> GSARNHTEDNSTEYYDYEEARCACPARHLNNTNGTVLKLLGCHYFCNGTLCTAPDGYPCYNLTAQQVRTLTTYPNTSCAVGVCMKGTCVKNGTMEQCFKTP;> ARGTNVGRECCLEYFKGAIP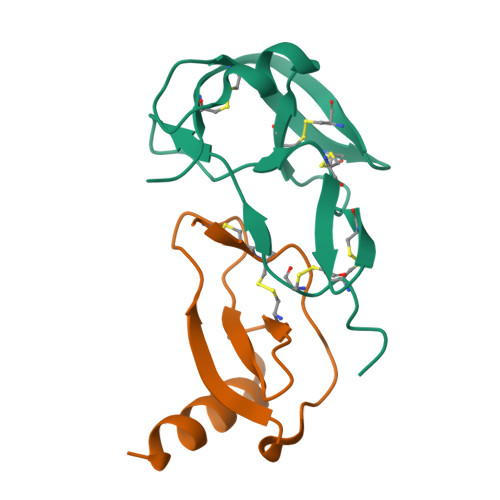LRKLKTWYQTSEDCSRDAIVFVTVQGRAICSDPNNKRVKNAVKYLQSLERS>[4x]GSHMASLTEIEHLVQSVCKSYRETCQLRLEDLLRQRSNIFSREEVTGYQRKSMWEMWERCAHHLTEAIQYVVEFAKRLSGFMELCQNDQIVLLKAGAMEVVLVRMCRAYN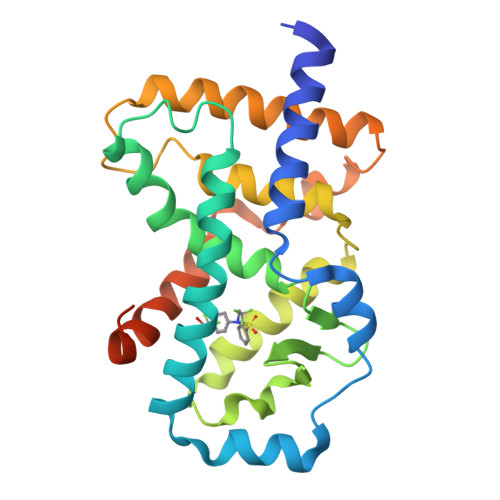ADNRTVFFEGKYGGMELFRALGCSELISSIFDFSHSLSALHFSEDEIALYTALVLINAHRPGLQEKRKVEQLQYNLELAFHHHLCKTHRQSILAKLPPKGKLRSLCSQHVERLQIFQHLHPIVVQAAFPPLYKELFS> EDMPVERILEAELAVEPKTETYVEANMGLNPSSPNDPVTNICQAADKQLFTLVEWAKRIPHFSELPLDDQVILLRAGWNELLIASFSHRSIAVKDGILLATGLHVHRNSAHSAGVGAIFDRVLTELVSKMRDMQMDKTELGCLRAIVLFNPDSKGLSNPAEVEALREKVYASLEAYCKHKYPEQPGRFAKLLLRLPALRSIGLKCLEHLFFFKLIGDTPIDTFLMEMLEA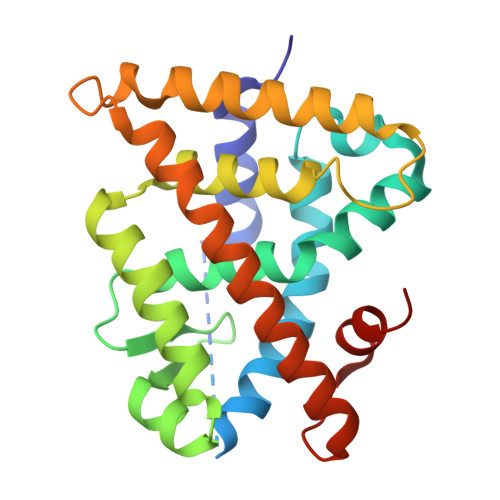PHQMT>AMDPEFMDAAIRQSLAKLGVQSTEIQASPVAGMKTVLTHSGVLYVTDDGKHIIQGPMYDVSGAHPVNVTNKLLMSQLNALEKEMIVYKAPDEKHVITVFTDITCGYCHKLHEEMKDYNALGITVRYLAFPRQGLESQAEQDMKSIWCAKDKNKAFDDAMAGKGVKPASCDVNIADHYALGV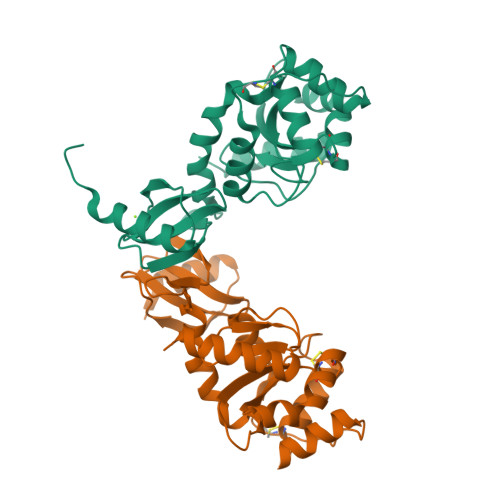QLGVSGTPAIVLSNGYVVPGYQGPKEMKAFLDEHQKQTSGK[2x]>PMILGYWNVRGLTHPIRLLLEYTDSSYEEKRYAMGDAPDYDRSQWLNEKFKLGLDFPNLPYLIDGSRKITQSNAIMRYLARKHHLCGETEEERIRADIVENQVMDNRMQLIMLCYNPDFEKQKPEFLKTIPEKMKLYSEFLGKRPWFAGDKVTYVDFLAYDILDQYHIFEPKCLDAFPNLKDFLARFE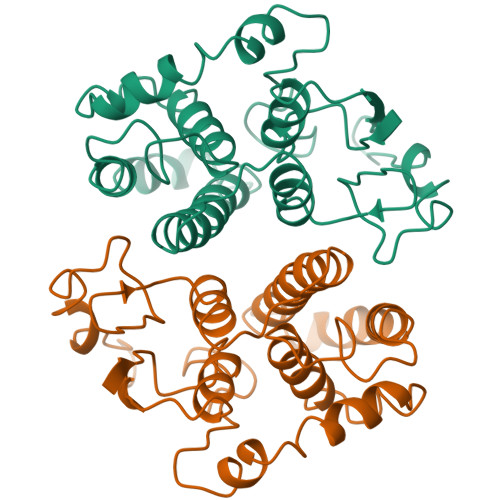GLKKISAYMKSSRYLSTPIFSKLAQWSNK[4x]> AEVTSIPTGCNALSGKIMSGFDANRFFTGDWYLTHSRDSEVPVRCEKYQTGSNLQLNFNGKNGDVKCSGSTVSGNQGFYSF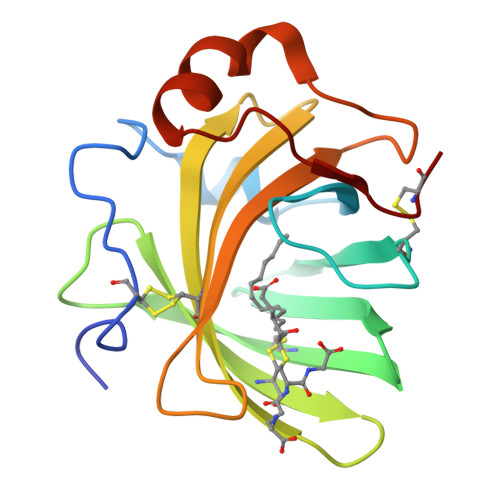QCTTTSGGSFTSYMAVVETDYANYALLYRCGLAGSTTPKDNFLLFNRQSSGEIPAGLSTKLNQLELTSLNKLGCS>MASNEGVENRPFPYLTVDADLLSNLRQSAAEGLFHSFDLLVGKDAREAGIKFEVLLGVYTNAIQYVRFLETALAVSCVNTEFKDLSRMTDGKIQFRISVPTIAHGDGRRPSKQRTFIVVKNCHKHHISTEMELSMLDLEILHSIPETPVEYAEYVGAVKTVASALQFGVDALERGLINTVLSVKLRHAPPMFILQTLADPTFTERGFSKTVKSDLIAMFKRHLLEHSFFLDRAENMGSGFSQYVRSRLSEMVAAVSGESVLKGVSTYTTAKGGEPVGGVFIVTDNVLRQLLTFLGEEADNQIMGPSSYASFVVRGENLVTAVSYGRVMRTFEHFMARIVDSPEKAGSTKSDLPAVAAGVEDQPRVPISAAVIKLGNHAVAVESLQKMYNDTQSPYPLNRRMQYSYYFPVGLFMPNPKYTTSAAIKMLDNPTQQLPVEAWIVNKNNLLLAFNLQNALKVLCHPRLHTPAHTLNSLNAAPAPRDRRETYSLQHRRPNHMNVLVIVDEFYDNKYAAPVTDIALKCGLPTEDFLHPSNYDLLRLELHPLYDIYIGRDAGERARHRAVHRLMVGNLPTPLAPAAFQEARGQQFETATSLAHVVDQAVIETVQDTAYDTAYPAFFYVVEAMIHGFEEKFVMNVPLVSLCINTYWERSGRLAFVNSFSMIKFICRHLGNNAISKEAYSMYRKIYGELIALEQALMRLAGSDVVGDESVGQYVCALLDPNLLPPVAYTDIFTHLLTVSDRAPQIIIGNEVYADTLAAPQFIERVGNMDEMAAQFVALYGYRVNGDHDHDFRLHLGPYVDEGHADVLEKIFYYVFLPTCTNAHMCGLGVDFQHVAQTLAYNGPAFSHHFTRDEDILDNLENGTLRDLLEISDLRPTVGMIRDLSASFMTCPTFTRAVRVSVDNDVTQQLAPNPADKRTEQTVLVNGLVAFAFSERTRAVTQCLFHAIPFHMFYGDPRVAATMHQDVATFVMRNPQQRAVEAFNRPEQLFAEYREWHRSPMGKYAAECLPSLVSISGMTAMHIKMSPMAYIAQAKLKIHPGVAMTVVRTDEILSENILFSSRASTSMFIGTPNVSRREARVDAVTFEVHHEMASIDTGLSYSSTMTPARVAAITTDMGIHTQDFFSVFPAEAFGNQQVNDYIKAKVGAQRNGTLLRDPRTYLAGMTNVNGAPGLCHGQQATCEIIVTPVTADVAYFQKSNSPRGRAACVVSCENYNQEVAEGLIYDHSRPDAAYEYRSTVNPWASQLGSLGDIMYNSSYRQTAVPGLYSPCRAFFNKEELLRNNRGLYNMVNEYSQRLGGHPATSNTEVQFVVIAGTDVFLEQPCSFLQEAFPALSASSRALIDEFMSVKQTHAPIHYGHYIIEEVAPVRRILKFGNKVVF[5x];>[5x]MARRLPKPTLQGRLEADFPDSPLLPKFQELNQNNLPNDVFREAQRSYLVFLTSQFCYEEYVQRTFGVPRRQRAIDKRQRASVAGAGAHAHLGGSSATPVQQAQAAASAGTGALASSAPSTAVAQSATPSVSSSISSLRAATSGATAAASAAAAVDTGSGGGGQPHDTAPRGARKKQ;>MKVQGSVDRRRLQRRIAGLLPPPARRLNISRGSEFTRDVRGLVEEHAQASSLSAAAVWRAGLLAPGEVAVAGGGSGGGSFSWSGWRPPVFGDFLIHASSFNNAEATGTPLFQFKQSDPFSGVDAVFTPLSLFILMNHGRGVAARVEAGGGLTRMANLLYDSPATLADLVPDFGRLVADRRFHNFITPVGPLVENIKSTYLNKITTVVHGPVVSKAIPRSTVKVTVPQEAFVDLDAWLSGGAGGGGGVCFVGGLGLQPCPADARLYVALTYEEAGPRFTFFQSSRGHCQIMNILRIYYSPSIMHRYAVVQPLHIEELTFGAVACLGTFSATDGWRRSAFNYRGSSLPVVEIDSFYSNVSDWEVIL[2x];>MDLKVVVSLSSRLYTDEIAKMQQRIGCILPLASTHGTQNVQGLGLGQVYSLETVPDYVSMYNYLSDCTLAVLDEVSVDSLILTKIVPGQTYAIKNKYQPFFQWHGTGSLSVMPPVFGREHATVKLESNDVDIVFPMVLPTPIAEEVLQKILLFNVYSRVVMQAPGNADMLDVHMHLGSVSYLGHHYELALPEVPGPLGLALLDNLSLYFCIMVTLLPRASMRLVRGLIRHEHHDLLNLFQEMVPDEIARIDLDDLSVADDLSRMRVMMTYLQSLASLFNLGPRLATAAYSQETLTATCWLR[4x];> MDVHIDNQVLSGLGTPLLVHLFVPDTVMAELCPNRVPNCEGAWCQTLFSDRTGLTRVCRVFAARGMLPGRPSHRGTFTSVPVYCDEGLPELYNPFHVAALRFYDEGGLVGELQIYYLSLFEGAKRALTDGHLIREASGVQESAAAMQPIPIDPGPPGGAGIEHMPVAAAQVEHPKTYDLKQILLEITQEENRGEQRLGHAGSPALCLGLRLRAGAETKAAAETSVSKHHPALENPSNIRGSAGGEGGGGRAGTGGTVGVGSGALSRVPVSFSKTRRAIRESRALVRGIAHIFSPHALYVVTYPELSAQGRLHRMTAVTHASPATDLAEVSILGAPEREFRFLISVALRISASFREKLAMQAWTAQQEIPVVIPTSYSRIYKNSDLIREAFFTVQTRVSWESCWVKATISNAPKTPDACLWIDSHPLYEEGASAWGKVIDSRPPGGLVGAASQLVALGTDGHCVHLATTSDGQAFLVLPGGFVIKGQLALTPEERGYILARHGIRREQ;>MALSGHVLIDPARLPRDTGPELMWAPSLRNSLRVSPEALELAEREAERARSERWDRCAQVLKNRLLRVELDGIMRDHLARAEEIRQDLDAVVAFSDGLESMQVRSPSTGGRSAPAPPSPSPAQPFTRLTGNAQYAVSISPTDPPLMVAGSLAQTLLGNLYGNINQWVPSFGPWYRTMSANAMQRRVFPKQLRGNLNFTNSVSLKLMTEVVAVLEGTTQDFFSDVRHLPDLQAALILSVAYLLLQGGSSHQQRPLPASREELLELGPESLEKIIADLKAKSPGGNFMILTSGNKEARQSIAPLNRQAAYPPGTFADNKIYNLFVGAGLLPTTAALNVPGAAGRDRDLVYRIANQIFGEDVPPFSSHQWNLRVGLAALEALMLVYTLCETANLAEAATRRLHLSSLLPQAMQRRKPAMASAGMPGAYPVQTLFRHGELFRFIWAHYVRPTVAADPQASISSLFPGLVLLALELKLMDGQAPSHYAINLTGQKFDTLFEIINQKLLFHDPAAMLAARTQLRLAFEDGVGVALGRPSPMLAAREILERQFSASDDYDRLYFLTLGYLASPVAPS[2x];>[2x]MSNGDWGQSQRTRGTGPVRGIRTMDVNAPGGGSGGSALRILGTASCNQAHCKFGRFAGIQCVSNCVLYLVKSFLAGRPLTSRPELDEVLDEGARLDALMRQSGILKGHEMAQLTDVPSSVVLRGGGRVHIYRSAEIFGLVLFPAQIANSAVVQSLAEVLHGSYNGVAQFILYICDIYAGAIIIETDGSFYLFDPHCQKDAAPGTPAHVRVSTYAHDILQYVGAPGAQYTCVHLYFLPEAFETEDPRIFMLEHYGVYDFYEANGSGFDLVGPELVSSDGEAAGTPGADSSPPVMLPFERRIIPYNLRPLPSRSFTSDSFPAARYSPAKTNSPPSSPASAAPASAAPASAAPASAAPASAAPASAAPASAAPASAAPASSPPLFIPIPGLGHTPGVPAPSTPPRASSGAAPQTPKRKKGLGKDSPHKKPTSGRRLPLSSTTDTEDDQLPRTHVPPHRPPSAARLPPPVIPIPHQSPPASPTPHPAPVSTIAPSVTPSPRLPLQIPIPLPQAAPSNPKIPLTTPSPSPTAAAAPTTTTLSPPPTQQQPPQSAAPAPSPLLPQQQPTPSAAPAPSPLLPQQQPPPSAARAPSPLPPQQQPLPSATPAPPPAQQLPPSATTLEPEKNHPPAADRAGTEISPSPPFGQQPSFGDDASGGSGLVRYLSDLEEPFLSMSDSEEAESDLASDIPTTEDEDMFEDEVFSNSLESGSSAPTSPITLDTARSQYYQTTFDIETPEMDFVPLESNIARIAGHTYQEQAIVYDPASNREVPEADALSMIDYLLVTVVLEQGLIRSRDRSSVLNLLEFLKDWSGHLQVPTLDLEQLLTSELNIQNLANMLSENKGRAGEFHKHLAAKLEACLPSLATKDAVRVDAGAKMLAEIPQLAESDDGKFDLEAARRRLTDLLSGGDQEAGEGGGEPEDNSIYRGPHVDVPLVLDDESWKRLLSLAEAARTAVARQQAGVDEEDVRFLALLTAIEYGAPPAASVPPFVHNVAVRSKNAALHVRRCTADIRDKVASAASDYLSYLEDPSLPTVMDFDDLLTHLRHTCQIIASLPLLNIRYTSIEWDYRELLYLGTALSDMSGIPWPLERVEEDDPSIAPLPEFETVAKKQKELETTRENEKRLRTILDDIEAMLGLAGVASAPGAPISPASPSATPANHDNPEATPPLADTAALTIPVIEKYIANAGSIVGAAKNPTYIRLRDTIQQIVRSKKYLMNILKSITFYTIDNYIASFEESIDHLYRDLPVLDPEVQDGIDRILDPMVSEALHTFEMGNRLTLEPARLVALQNFATHSTLKETAAAVNLLPGLLAVYDATITGQAPEDALRLLSGLQNQLSQTLIPGKLKKRFLSYLQKLKNNNNDQLRQKEVQAWRLEAEGFKPATEEQLEAFLDTAPNKELKRQYEKKLRQLMETGRKEKEKLREQEDKERQERRAREANEAWARIRKALGARPEPAPTSPDDWNTLLASLLPDNTDSAAAAAAAVARNTDILDSLTQILAAMLLGITRVRRERLRSLLVDDGGAAERMEAAEPGWFTDIETGPLARLDAWPATPAATAKEGGGGRGAEEAAGALFRARTAADAIRSALAQTRQALQSPDMKSAVVNTDLEAPYAEYERGLAGLLEKRRAAEAALTAIVSEYVDRTLPEATNDPGQANLPPPPTIPQA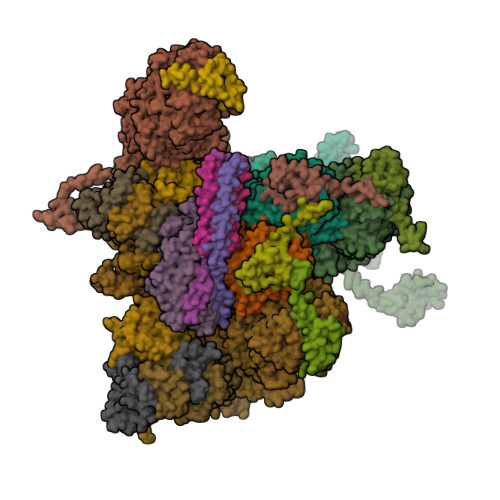TAPPRLASDSALWPKKPQLLTRRERDDLLQATGDFFSELLTEAEAAEVRALEEQVRESQTLMAKAHEMAASTRRGFHTALEAVLSRSRDEAPDDELRSLLPSPPKAPVQAPLEAALARAAAGNGSWPYRKSLAAAKWIRGICEAVRGLSEGALALAGGAGAWLNLAAAADGEIHELTRLLEVEGMAQNSMDGMEELRLALATLDPKRVAGGKETVADWKRRLSRLEAIIQEAQEESQLQGTLQDLVTQARGHTDPRQLKIVVEAARGLALGASAGSQYALLKDKLLRYASAKQSFLAFYETAQPTVFVKHPLTNNLPLLITISAPPTGWGNGAPTRRAQFLAAAGPAKYAGTLWLETESPCDPLNPAYVSADTQEPLNYIPVYHNFLEYVMPTVLENPEAFSLTPAGRPQAIGPPQDDQERRRRTLASVASARLSAAAADSYWDTWPDVESNAGELLREYVSAPKALMEDLADNPIVAMTLLAHASLIASRNHPPYPAPATDREVILLEQREMMALLVGTHPAYAAAFLGAPSFYAGLGLVSALARDGGLGDLLSDSVLTYRLVRSPASGRGGMPSTTRGSNDGEDARRLTRHRIAGPPTGFIFFQDAWEEMDTRAALWPHPEFLGLVHNQSTARARACMLLLARRCFAPEALQQLWHSLRPLEGPVAFQDYLRDFVKQAYTRGEELPRAEGLEVPRETPSSYGTVTGRALRNLMPYGTPITGPKRGSGDTIPVSVFEAAVAAAFLGRPLTLFVSSQYLFNLKTLGQVRVVAPLLYCDGHSEPFRSLVETISLNFLQDLDGYSESFEPEMSIFARQAVWLRELLTEARAAKPKEARPPTVAILANRKNIIWKCFTYRHNLPDVQFYFNAAGASRWPTDVLNPSFYEHEDPPLPVGYQLPPNPRNVQELFSGFPPRVGHGLVSGDGFQSADNTPASSDRLQQLGGGETDQGEKGSTTAESEASGPPSPQSPLLEKVAPGRPRDWLSPTSSPRDVTVTPGLAAPITLPGPRLMARPYFGAETRASESPDRSPGSSPRPWPKDSLELLPQPAPQQPPSSPWASEQGPIVYTLSPHSTPSTASGSQKKHTIQIPGLVPSQKPSYPPSAPYKPGQSTGGIAPTPSAASLTTFGLQPQDTQASSQDPPYGHSIMQREKKQQGGREEAAEIRPSATRLPTAVGLRPRAPVVAAGAAASATPAFDPGEAPSGFPIPQAPALGSGLAAPAHTPVGALAPRPQKTQAQRPQDAAALPTPTIKAVGARPVPKATGALAAGARPRGQPTAAPPSAASPPRVSLPVRSRQQQSPAIPLPPMHSGSEPGARPEVRLSQYRHAGPQTYTVRKEAPPSAASQLPKMPKCKDSMYYPPSGSARYPAPFQALSFSQSVASPAPSSDQTTLLWNTPSVVTQFLSIEDIIREVVTGGSTSGDLVVPSGSPSSLSTAAPEQDLRYSLTLSQASRVLSRFVSQLRRKLERSTHRLIADLERLKFLYL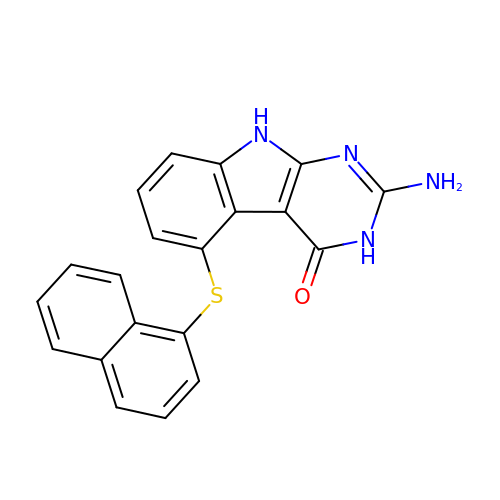2-Amino-5-(1-naphthylsulfanyl)-3,9-dihydro-4H-pyrimido[4,5-b]indol-4-one | C20 H14 N4 O S | NSASWBYEPOLHJW-UHFFFAOYSA-N> MGSSHHHHHHSSGRENLYFQGHMNGDQNSDVYAQEKQDFVQHFSQIVRVLTEDEMGHPEIGDAIARLKEVLEYNTIGGKYNRGLTVVVAFRELVEPRKQDADSLQRAWTVGWCVELLQAFFLVADDIMDSSLTRRGQICWYQKPGVGLDAINDANLLEACIYRLLKLYCREQPYYLNLIELFLQSSYQTEIGQTLDLLTAPQGNVDLVRFTEKRYKSIVKYGTAFYSFYLPIAAAMYMAGIDGEKEHANAKKILLEMGEFFQIQDDYLDLFGDPSVTGKIGTDIQDNKCSWLVVQCLQRATP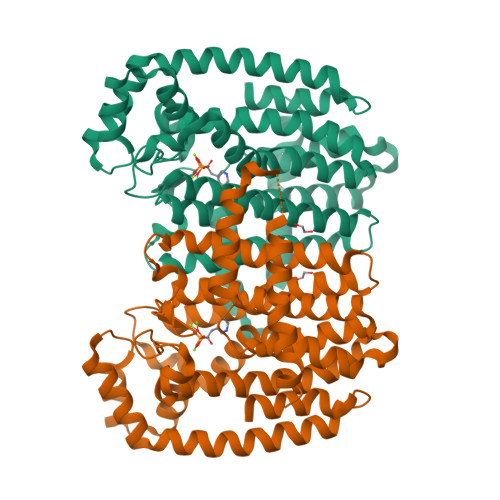EQYQILKENYGQKEAEKVARVKALYEELDLPAVFLQYEEDSYSHIMALIEQYAAPLPPAVFLGLARKIYKRRK> G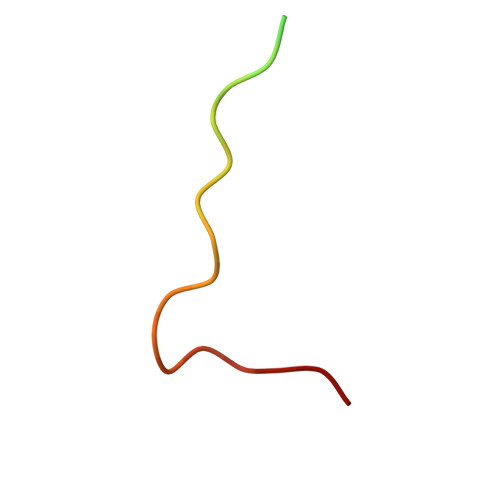PGSGRTEGQLMRYQHPPEYGAARPA> MASNLVEMFNAALNWVTMILESPSARVVLFGVPIRGHFFVEGLLGVVIIILLTRKSYKPPKRPLTEQEIDELCDEWVPEPLIPPITEDMKHEPPVLESAAGPHTTVNGKDVVNFASANYLGLIGHEKLLESCTSALEKYGVGSCGPRGFYGTIDVHLDCETRISKFLGTPDSILYSYGLSTMFSTIPCFCKKGDVIVADEGVHWGIQNGLQLSRSTIVYFKHNDMESLRITLEKIMTKYKRSKNLRRYIVAEAVYQNSGQIAPLDEIVKLKEKYRFRVILDESNSFGVLGRSGRGL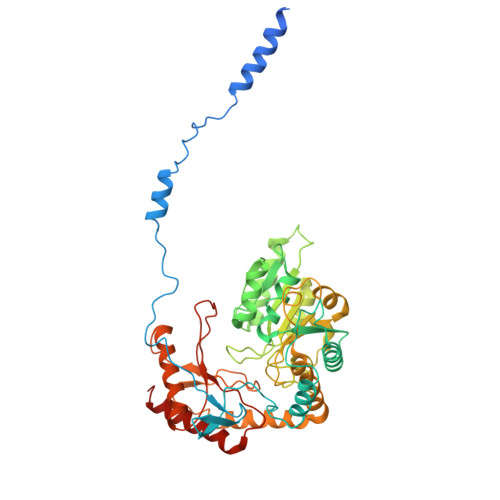AEHHSVPIEKIDVVTAAMGHALATEGGFCTGNARIIDYQRLSSSGYVFSASLPPYLASAAITAIDVIDQNPDMLVKLKQNVALLWKGLSDIKGMSLTSNRESPIVFLKLEKSSGSAKDDLLLLEKMADRALKEDSLLVVSSKRSFLDKCRLPVGIKLYVSAGHSESDLLKASESLKRLASELLLKS> GSHMDKLPIEETLEDSPQTRSLLGVFEEDATAISNYMNQLYQAMHRIYDAQNELSAATHLTSKLLKEYEKQRFPLGGDDE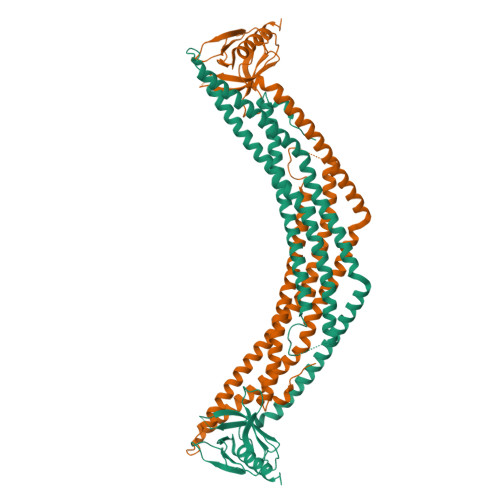VMSSTLQQFSKVIDELSSCHAVLSTQLADAMMFPITQFKERDLKEILTLKEVFQIASNDHDAAINRYSRLSKKRENDKVKYEVTEDVYTSRKKQHQTMMHYFCALNTLQYKKKIALLEPLLGYMQAQISFFKMGSENLNEQLEEFLANIGTSVQNVRREMDSDIETMQQTIEDLEVASDPLYVPDPDPTKFPVNRNLTRKAGYLNARNKTGLVSSTWDRQFYFTQGGNLMSQARGDVAGGLAMDIDNCSVMAVDCEDRRYCFQITSFDGKKSSILQAESKKDHEEWICTINNISKQIYLSENPEE> UCCCAGUCCACCG;> CGGUGAGAA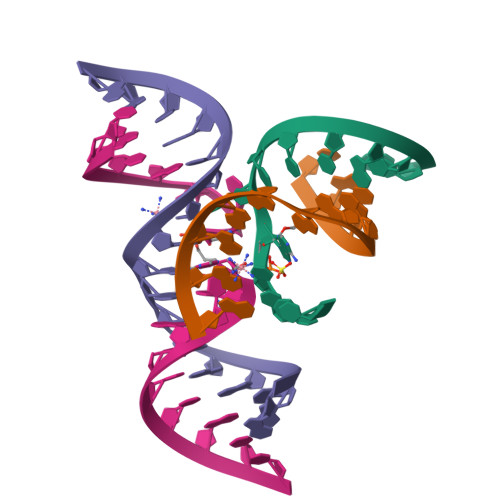GGG;> GGCAGAGAAACACACGA;> UCGUGGUAXAUUACCUGCC>[6x]MGSDKIHHHHHHENLYFQGMQCPIED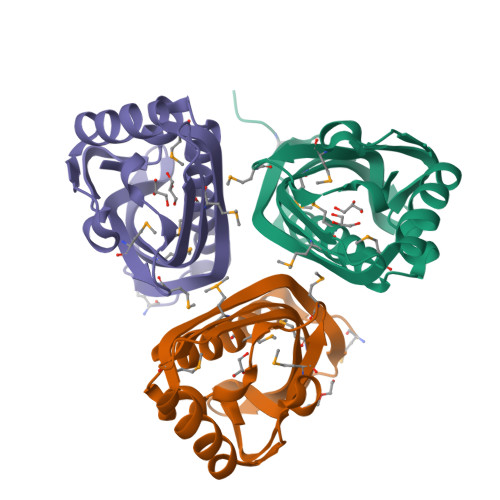RLAIQDLMIAYAHAVDTVSDIDAVLDVFTEDAVFDLSGIGLTPQVGHAGIREFFTNVFANMSHHAHYLTNFAVTGYEGDTASMRAYVIGMGVGKDGRAVTVNGRYFFEVRRTEKGWKATRYTMDFLMPLSGTLDNAK>MGSKQNQKSVNKHDKEALYRYYTGKTMEMKNISALKHGKNNLRFKFRGIKIQVLLPGNDKSKFQQRSYEGLDVFFVQEKRDKHDIFYTVGGVIQNNKTSGVVSAPILNISKEKGEDAFVKGYPYYIKKEKITLKELDYKLRKHLIEKYGLYK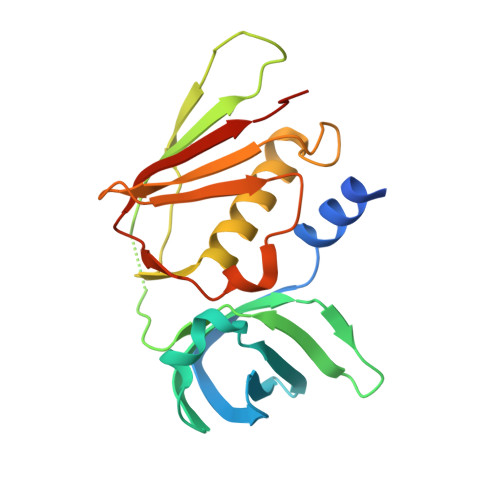TISKDGRVKISLKDGSFYNLDLRSKLKFKYMGEVIESKQIKDIEVNLKLEHHHHHH[2x]> MISARAVHRFLRNPNLETGAAFRAGTRFDPFKNTLTVLKDPQNGRTLYLIGTTNSSTLLANRTKDLVQKEKPDAVFVQTNKEWWNLAKNIQDVKCQQELNRYNDLLSQAYTLSLDNTIRNLVFKAKFYSWLFVINWFKAFPDDFHPFIPGLEMKFAI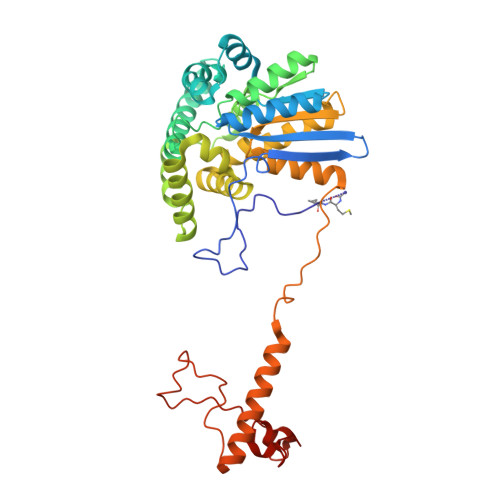EEANKQNIPVVLGGLEVDDVTLSALKVEPRLDPFSQLYYGYRALHNSFWRREHFDNYATLDVVGGEAYAESMDRFRTNWFVKYFEKLAPYQKKIIVDQKDLDLFYALYRDTPGKKIVAVVNQWHVPGIENHWKSATNTHEPLKAINPIGDMDINKYMESQLVNDTLRAFVSKVGKTEPATWKNYSTIYHKDNYEAERVRHVAFVDHKDPHMYHGLPQDYDDNIKPKHH>MDNGELISIIVPVYNVEKYLKRCLDSLLRQTYKNFEIILINDGSTDNSSIICEEYAKIDNRIQILHQTNAGPSAARNAGITYASGKYIT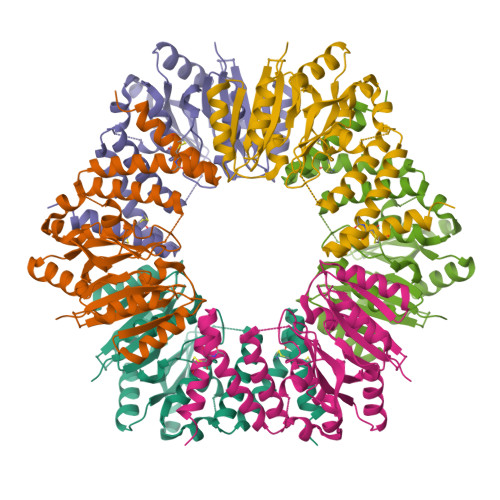FVDSDDFVEEFYLEHLYRALVDNGSDISVCNFNSFNEDRQSFLFSITKEKYFCKNYTIAEWMDLESSANNNLFLTFTFSPTKLFKAELFEGIRFPLGRLREDDATIYRLYLKASQITFINEGSYYYSQRSEGLSRTRMLDDISSMISNAEERIALLASMGYDLTEQIKSYKGRLKKCCEDALRNGQIELYQQCCNKLDLIENYPKEK[3x]> PNLTEISKKITESNAVVLAVKEVETLLASIDELATKAIGKKIGNNGLEANQSKNTSLLSGAYAISDLIAEKLN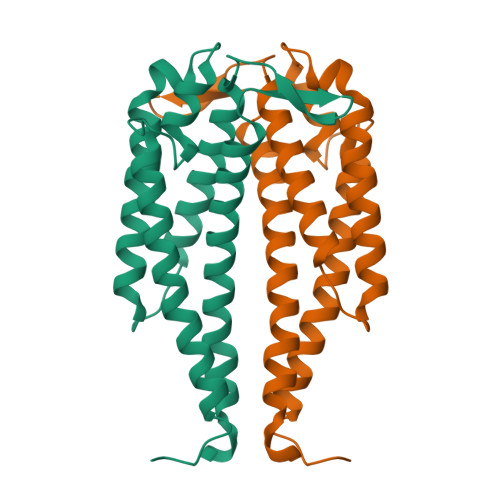VLKNEELKEKIDTAKQCSTEFTNKLKSEHAVLGLDNLTDDNAQRAILKKHANKDKGAAELEKLFKAVENLSKAAQDTLKNAVKELTSPIVA> MEINVTAPALLTDEHILQPFDCGNEVLSNWLRGRAMKNQMLNASRTFVICLEDTLRIVGYYSLATGSVTHAELGRSLRHNMPNPVPVVLLGRLAVDVCTRGH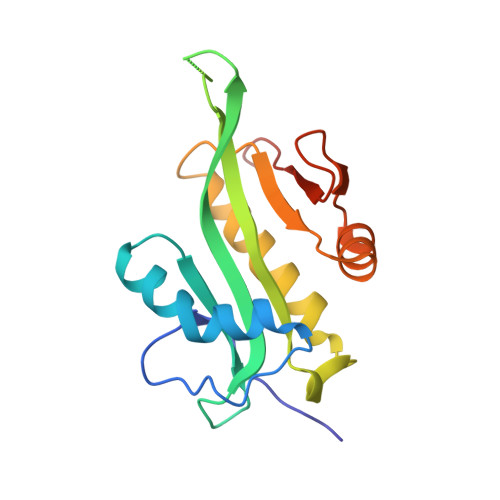GFGKWLLSDAIHRVVNLADQVGIKAVMVHAIDDDARAFYERFGFVQSVVAPNTLFYKVLEHHHHHH>[2x]MLQKKIEEIAAKYKHSVVKKCCYDGACVNND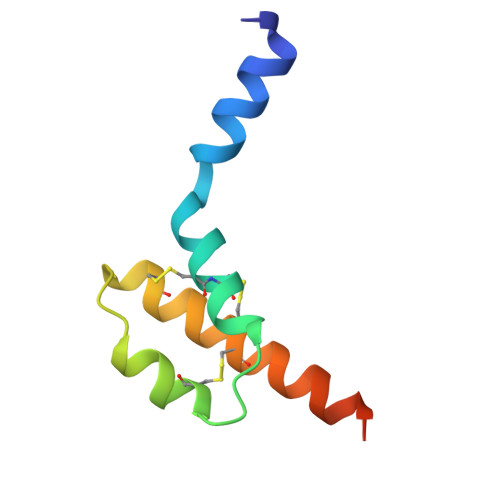ETCEQRAARISLGPRCIKAFTECCVVASQLRANISHKDMQLG>[8x]SSEQLQALLLEEVMNSSTLSQEVSDLVEMIWAEALGHLEHMLLKPVNRISLNDVSKAEGILLLVKAALKNGETAEQLQKMMTEFYRLIPHKGTMPKEVNLGLLAKKADLCQLIRDMVNVCETNLSKPNPPSLAKYRALRCKIEHVEQNTEEFLRVRKEVLQNHHSKSPVDVLQIFRVGRVNETTEFLSKLGNVRPLLHGSPVQNIVGILCRGLLLPKVVEDRGVQRTDVGNLGSGIYFSDSLSTSIKYSHPGETDGTRLLLICDVALGKCMDLHEKDFSLTEAPPGYDSVHGVSQTASVTTDFEDDEFVVYKTNQVKMKYIIKFSMPGDQIKD

PARP4 is an ADP-ribosyltransferase that resides within the vault ribonucleoprotein organelle. PARP4 is an ADP-ribosyltransferase that uses NAD+ as a substrate to synthesize ADP-ribose modifications on molecules. The PARP1-homology region of PARP4 includes a BRCT fold, a WGR domain, and the catalytic (CAT) domain. However, PARP3 and PARP4 contain the catalytic triad H-Y-E but are considered MARylation enzymes, indicating that other structural features are important determinants of catalytic output.

We reasoned that the bound EB47 molecule could potentially influence the positioning of the HD relative to the ART, thus we sought a PARP4 CAT structure with no compound in the active site. Crystals of the PARP4 catalytic domain alone diffracted to 4.2 Å and belonged to space group P212121 with eight molecules in the asymmetric unit. The refined structure has a crystallographic R/RFREE of 0.277/0.331. Despite the modest resolution, the structure clearly indicated that PARP4 HD adopts a similar orientation relative to the ART regardless of active site occupancy. The HD conformation was consistently open in all copies of the CAT domain within the two crystal types (10 copies total). Since these copies occupy different crystal environments, we deem it unlikely that the open HD conformation is a product of crystallization. Here, we have determined crystal structures of the PARP4 catalytic region that indicate that PARP4 indeed contains an HD domain, but the HD conformation is quite distinct from PARP1 and biochemical analysis indicates a more ‘open’ PARP4 ART active site relative to PARP1. In the collection of PARP4 structures determined in this study, the N-terminal helix adopts several conformations relative to the rest of the HD/ART folds, suggesting that it is flexibly attached to the catalytic domain. In contrast to PARP1, the PARP4 catalytic domain was clearly active, consistent with the structural observation of an open and accessible active site.> MFERFTDRARRVVVLAQEEARMLNHNYIGTEHILLGLIHEG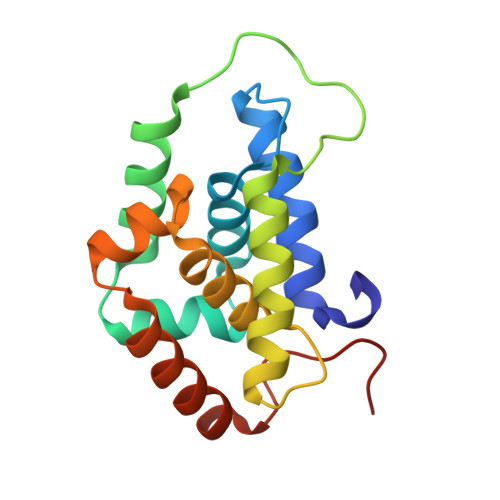EGVAAKSLESLGISLEGVRSQVEEIIGQGQQAPSGHIPFTPRAKKVLELSLREALQLGHNYIGTEHILLGLIREGEGVAAQVLVKLGAELTRVRQQVIQLLSGYQGKLEHHHHHH> KA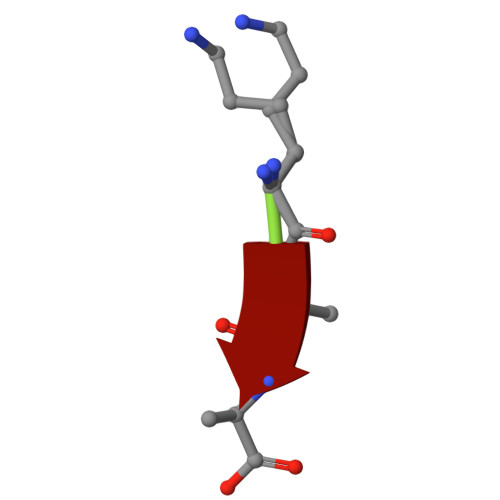A>PRVDPRV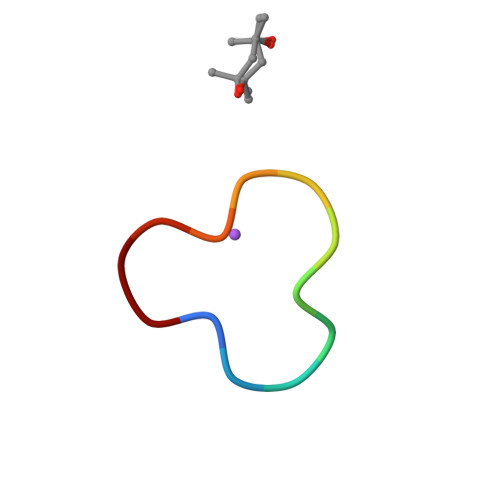DPRVD[4x]> MIRRRVCDGARLAPNIRATFSAVRYQSGLHTFIRDSKPSNFSSVRRSENANGDATASPGATAGENPASSGDWASHMQRELFGEVDPLGGQAHKDYYRDVTRGYSPQYAPRNFANGGAVAYPHIQSPYEYEEAAHRRVWLDHDVDRMREEFTQHRASLRSLASAQEREELLRSRAAEYQVANTVHESESVHPIQQLYNSGGTSRSALKQQAVADRYSIAEQHSPLPLTTGVDRDALDEAQRTKDRILNDSFTAENLLITHGLREKEKHDFTILQRTVRIPFQGYDMDRFLAQQKGTPYGAQQLPPNVVPSSMEEAQRTLRGSSATATPLVDAVAQKVYARNTVVDRPAIGEQLTEQIINIMRASRTTAEQQREEERAQRFGLGRQGALVQDGGPDQRTLKKHTNDERIVDAMLFQQNAYRKTPTDEHWNPYIRRSTENGVGHLLQNKFDIMRREDRLSKGEQDLTERNTIHYGVPIQQIVDEFVFRHRNARGERPLDYFKPFPNFRALRLNRMYRDVEGFSLMKQRPEFLEWELFTRYRQHHQQRRRLALLHGLEPVANETAQERDTRRHRLDEICERTPFDEREMRVNDDEMRVSVETLRSWFGVYMLPSPTVVNAV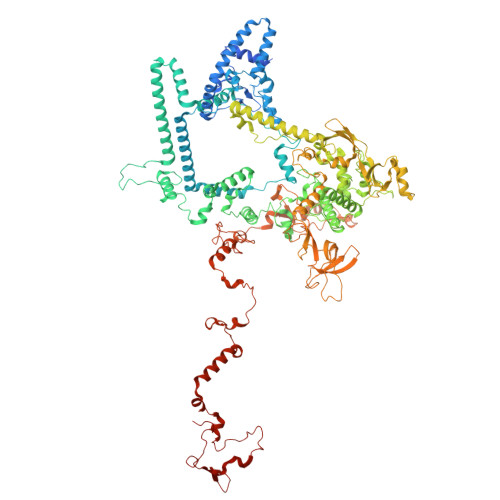LGGSASVNLHLYHLADEMGTADTREHVLSSRYLNRLLLLESYQNRVGRGFMNHVVGRAPEPVVPHEQPQEVLRHFSAEERAMYEQHVKEQTSRQLGEWERAMKRRRWLTDHQQYGHVVSHGLETSVVDLSHTETGAVLTVSTKAYEQEIEAVRMKTNATIKVDGMVYNLLPNSERRVVPLTVQLDSGEKIDMTSEDFDRCELEAFPRNLNHALNYGIANYAYNRGNYVETQDSIWEEQTASGQEGWSPATHADGLREGLPVRARRPIFSSSAEQRIAGGPQRAVIIQYHHQPFFNPEPRLVKVAFQCDGTIMEVPISDVMIWQRRYHGPERTVGDESRRYNPAAMRRYVDVTDPFNEKTSNTEHFLDKYEPKRNADTVADKYRTTKQITEIDKWTRYDSARADNYRPLSISHRRDYIRMGYIPRYTPWEWIAIQEADQPLIAEQIRQDNIGTSYFFSLNRYWRYKASPHGYIRHFENEVRDLLQYVDGVTPWKQAQKIRTYWEVRSHHPMPQFNRPEVAMHRNTVGLLPAHMWETDKKTGKVKSVKDSVRDYQTKTPYPKWVQL> MGSSHHHHHHSQDPNSMPDNTIQWDKDADGIVTLTMDDPSGSTNVMNEAYIESMGKAVDRLVAEKDSITGVVVASAKKTFFAGGDVKTMIQARPEDAGDVFNTVETIKRQLRTLETLGKPVVAAINGAALGGGLEIALACHHRIAADVKGSQLGLPAVTLGLLPGGGGVTRTVRMFGIQNAFVSVLAQGTRFKPAKAKEIGLVDELVATVEELVPAAKAWIKEELKANPDGAGVQPWDKKGYKMPGGTPSSPGLAAILPSFPSNLRKQLKGAPMPAPRAILAAAVEGAQVDFD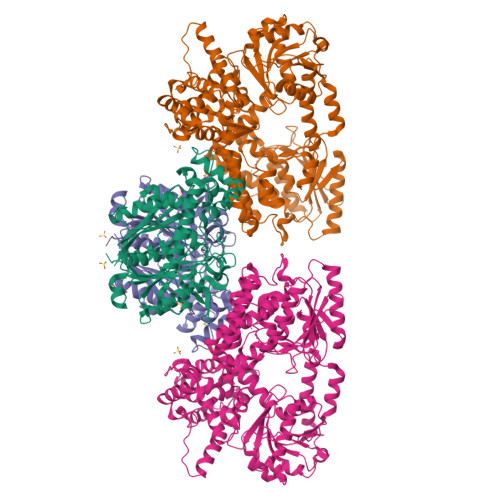TASRIESRYFASLVTGQVAKNMMQAFFFDLQAINAGGSRPEGIGKTPIKRIGVLGAGMMGAGIAYVSAKAGYEVVLKDVSLEAAAKGKGYSEKLEAKALERGRTTQERSDALLARITPTADAADFKGVDFVIEAVFENQELKHKVFGEIEDIVEPNAILGSNTSTLPITGLATGVKRQEDFIGIAFFSPVDKMPLVEIIKGEKTSDEALARVFDYTLAIGKTPIVVNDSRGFFTSRVIGTFVNEALAMLGEGVEPASIEQAGSQAGYPAPPLQLSDELNLELMHKIAVATRKGVEDAGGTYQPHPAEAVVEKMIELGRSGRLKGAGFYEYADGKRSGLWPGLRETFKSGSSQPPLQDMIDRMLFAEALETQKCLDEGVLTSTADANIGSIMGIGFPPWTGGSAQFIVGYSGPAGTGKAAFVARARELAAAYGDRFLPPESLLS;> MSEEAFIYEAIRTPRGKQKNGSLHEVKPLSLVVGLIDELRKRHPDLDENLISDVILGCVSPVGDQGGDIARAAVLASGMPVTSGGVQLNRFAASGLEAVNTAAQKVRSGWDDLVLAGGVESMSRVPMGSDGGAMGLDPATNYDVMFVPQSIGADLIATIEGFSREDVDAYALRSQQKAAEAWSGGYFAKSVVPVRDQNGLLILDHDEHMRPDTTKEGLAKLKPAFEGLAALGGFDDVALQKYHWVEKINHVHTGGNSSGIVDGAALVMIGSAAAGKLQGLTPRARIVATATSGADPVIMLTGPTPATRKVLDRAGLTVDDIDLFELNEAFASVVLKFQKDLNIPDEKLNVNGGAIAMGHPLGATGAMILGTMVDELERRNARRALITLCIGGGMGVATIIERV> MCWAAAIPIAISGAQAISGQNAQAKMIAAQTAAGRRQAMEIM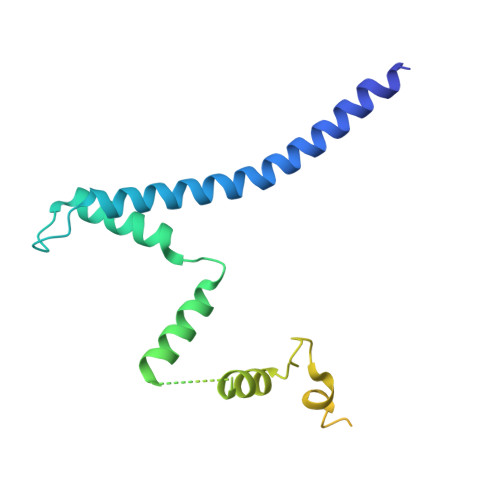RQTNIQNADLSLQARSKLEEASAELTSQNMQKVQAIGSIRAAIGESMLEGSSMDRIKRVTEGQFIREANMVTENYRRDYQAIFAQQLGGTQSAASQIDEIYKSEQKQKSKLQMVLDPLAIMGSSAASAYASGAFDSKSTTKAPIVAAKGTKTGR> GPLGSMRRSKADVERYIASVQGSTPSPRQKSIKGFYFAKLYYEAKEYDLAKKYICTYINVQERDPKAHRFLGLLYELEENTDKAVECYRR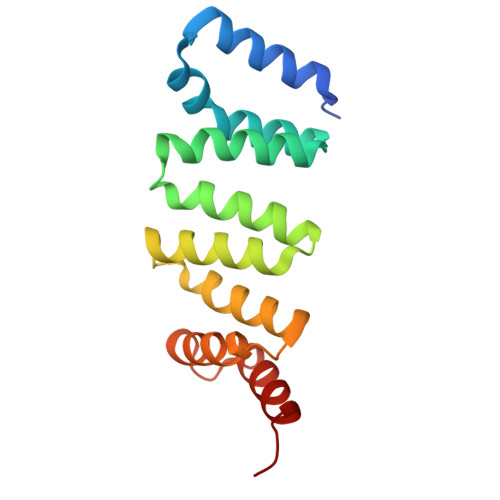SVELNPTQKDLVLKIAELLCKNDVTDGRAKYWVERAAKLFPGSPAVYKLKEQLLDCEGED> GP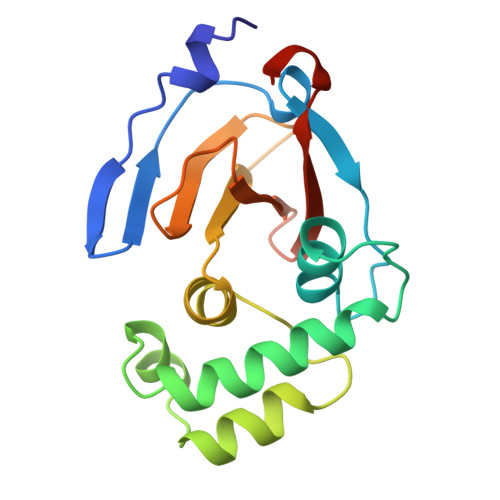MDFLRSLDWTQVIAGQYVSNPRFNISDYFEIVRQPGDGNCFYHSIAELTMPNKTDHSYHYIKRLTESAARKYYQEEPEARLVGLSLEDYLKRMLSDNEWGSTLEASMLAKEMGITIIIWTVAASDEVEAGIKFGDGDVFTAVNLLHSGQTHFDALRILPQFETDTREAL>MSQFMNLEGKVALVTGASRGIGKAIAELLAERGAKVIGTATSESGAQAISDYLGDNGKGMALNVTNPESIEAVLKAITDEFGGVDILVNNAGITRDNLLMRMKEEEWSDIMETNLTSIFRLSKAVLRGMMKKRQGRIINVGSVVGTMGNAGAANYAAAKAGVIGFTKSMAREVASRGVTVNTVAPGFIETDMTKALNDEQRTATLAQVPAGRLGDPREIASAVAFLASPEAAYITGETLHVN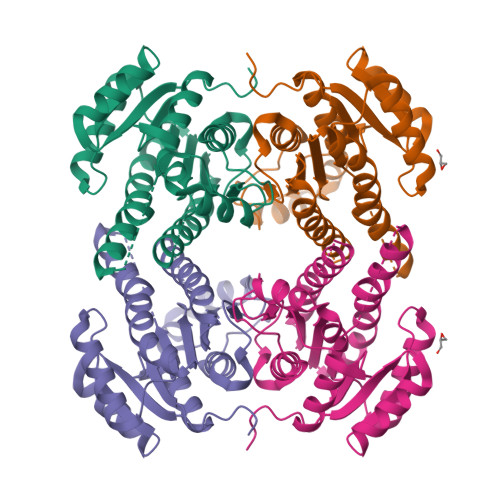GGMYMI[2x]> MKCLVTGGNVKVLGKAVHSLS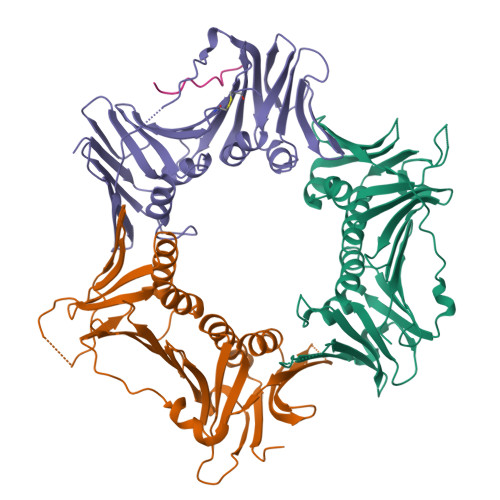RIGDELYLEPLEDGLSLRTVNSSRSAYACFLFAPLFFQQYQAATPGQDLLRCKILMKSFLSVFRSLAMLEKTVEKCCISLNGRSSRLVVQLHCKFGVRKTHNLSFQDCESLQAVFDPASCPHMLRAPARVLGEAVLPFSPALAEVTLGIGRGRRVILRSYHEEEADSTAKAMVTEMCLGEEDFQQLQAQEGVAITFCLKEFRGLLSFAESANLNLSIHFDAPGRPAIFTIKDSLLDGHFVLATLSDTDS;> MHHHHHHKFRAKIVDGACLNHFTRISNMIAKLAKTCTLRISPDKLNFILCDKLANGGVSMWCELEQENFFNEFQMEGVSAENNEIYLELTSENLSRALKTAQNARALKIKLTNKHFPCLTVSVELLSMSSSSRIVTHDIPIKVIPRKLWKDLQEPVVPDPDVSIYLPVLKTMKSVVEKMKNISNHLVIEANLDGELNLKIETELVCVTTHFKDLGNPPLASESTHEDRNVEHMAEVHIDIRKLLQFLAGQQVNPTKALCNIVNNKMVHFDLLHEDVSLQYFIPALS;> MPLLTQQIQDEDDQYSLVASLDNVRNLSTILKAIHFREHATCFATKNGIKVTVENAKCVQANAFIQAGIFQEFKVQEESVTFRINLTVLLDCLSIFGSSPMPGTLTALRMCYQGYGYPLMLFLEEGGVVTVCKINTQEPEETLDFDFCSTNVINKIILQSEGLREAFSELDMTSEVLQITMSPDKPYFRLSTFGNAGSSHLDYPKDSDLMEAFHCNQTQVNRYKISLLKPSTKALVLSCKVSIRTDNRGFLSLQYMIRNEDGQICFVEYYCCPDEEVPESES;> SKPIDHSTITSWVSPDFDTA> GSHMLRPVETPTREIKKLDGLWAFSLDRENCGIDQRWWESALQESRAIAVPGSFNDQFADADIRNYAGNVWYQREVFIPKGWAGQRIVLRFDAVTHYGKVWVNNQEVMEHQGGYTPFEADVTPYVIAGKSVRITVCVNNELNWQTIPPGMVITDENGKKKQSYFHDFFNYAGIHRSVMLYTTPNTWVDDITVVTHVAQDCNHAS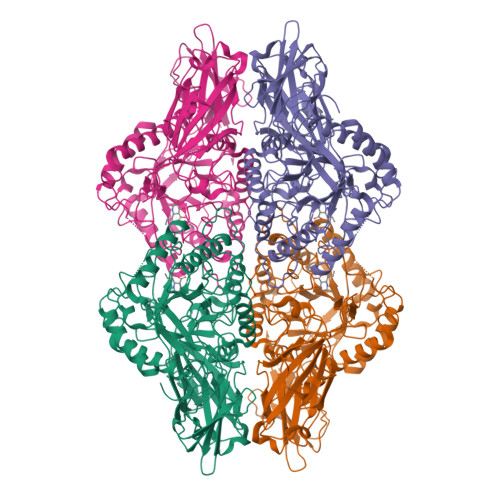VDWQVVANGDVSVELRDADQQVVATGQGTSGTLQVVNPHLWQPGEGYLYELCVTAKSQTECDIYPLRVGIRSVAVKGEQFLINHKPFYFTGFGRHEDADLRGKGFDNVLMVHDHALMDWIGANSYRTSHYPYAEEMLDWADEHGIVVIDETAAVGFNLSLGIGFEAGNKPKELYSEEAVNGETQQAHLQAIKELIARDKNHPSVVMWSIANEPDTRPQGAREYFAPLAEATRKLDPTRPITCVNVMFCDAHTDTISDLFDVLCLNRYYGWYVQSGDLETAEKVLEKELLAWQEKLHQPIIITEYGVDTLAGLHSMYTDMWSEEYQCAWLDMYHRVFDRVSAVVGEQVWNFADFATSQGILRVGGNKKGIFTRDRKPKSAAFLLQKRWTGMNFGEKPQQGGKQ;> MLRPVETPTREIKKLDGLWAFSLDRENCGIDQRWWESALQESRAIAVPGSFNDQFADADIRNYAGNVWYQREVFIPKGWAGQRIVLRFDAVTHYGKVWVNNQEVMEHQGGYTPFEADVTPYVIAGKSVRITVCVNNELNWQTIPPGMVITDENGKKKQSYFHDFFNYAGIHRSVMLYTTPNTWVDDITVVTHVAQDCNHASVDWQVVANGDVSVELRDADQQVVATGQGTSGTLQVVNPHLWQPGEGYLYELCVTAKSQTECDIYPLRVGIRSVAVKGEQFLINHKPFYFTGFGRHEDADLRGKGFDNVLMVHDHALMDWIGANSYRTSHYPYAEEMLDWADEHGIVVIDETAAVGFNLSLGIGFEAGNKPKELYSEEAVNGETQQAHLQAIKELIARDKNHPSVVMWSIANEPDTRPQGAREYFAPLAEATRKLDPTRPITCVNVMFCDAHTDTISDLFDVLCLNRYYGWYVQSGDLETAEKVLEKELLAWQEKLHQPIIITEYGVDTLAGLHSMYTDMWSEEYQCAWLDMYHRVFDRVSAVVGEQVWNFADFATSQGILRVGGNKKGIFTRDRKPKSAAFLLQKRWTGMNFGEKPQQGGKQ> MSAVKAARYGKDNVRVYKVHKDEKTGVQTVYEMTVCVLLEGEIETSYTKADNSVIVATDSIKNTIYITAKQNPVTPPELFGSILGTHFIEKYNHIHAAHVNIVCHRWTRMDIDGKPHPHSFIRDSEEKRNVQVDVVEGKGIDIKSSLSGLTVLKSTNSQFWGFLRDEYTTLKETWDRILSTDVDATWQWKNFSGLQEVRSHVPKFDATWATAREVTLKTFAEDN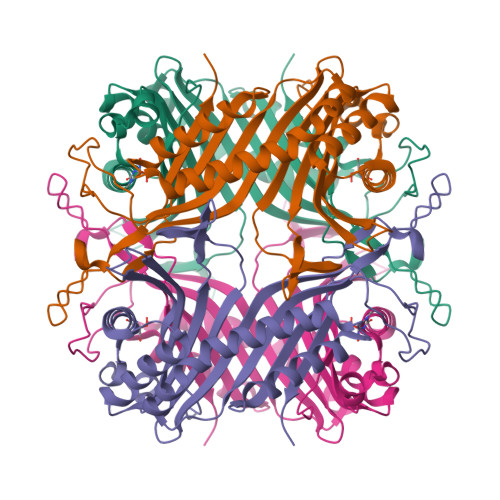SASVQATMYKMAEQILARQQLIETVEYSLPNKHYFEIDLSWHKGLQNTGKNAEVFAPQSDPNGLIKCTVGRSSLKSKL>[2x]QGMSDAFTDVAKMKKIKEEIKAHEGQVVEMTLENGRK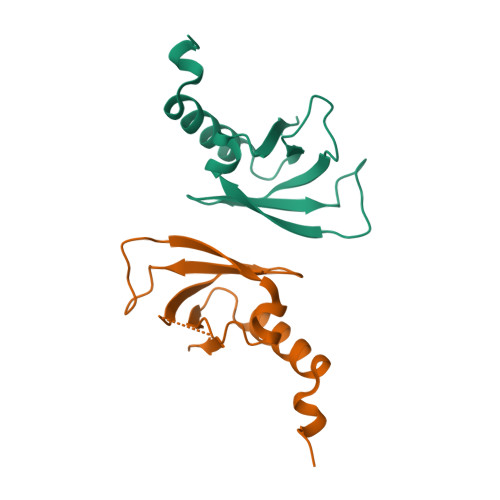RQKNRLGKLIEVYPSLFIVEFGDVEGDKQVNVYVESFTYSDILTEKNLIHYLD2-[4-[(2~{R})-4-[4-(6-carboxy-1~{H}-benzimidazol-2-yl)phenoxy]-2-oxidanyl-butoxy]phenyl]-1~{H}-benzimidazole-5-carboxylic 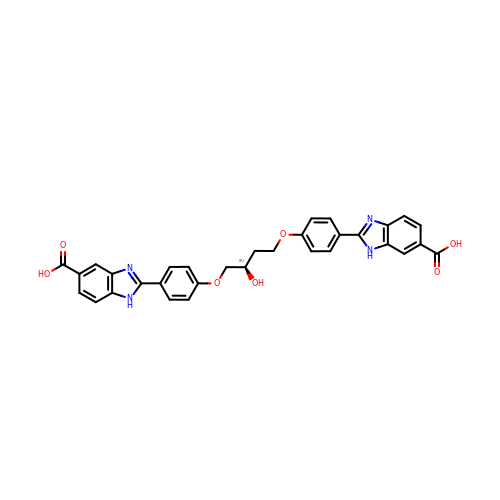acid | C32 H26 N4 O7 | QQYJHKTWHJAQJJ-JOCHJYFZSA-N>AMRQCAIYGKGGIGKSTTTQNLVAALAEMGKKVMIVGCDPKADSTRLILHSKAQNTIMEMAAEAGTVEDLELEDVLKAGYG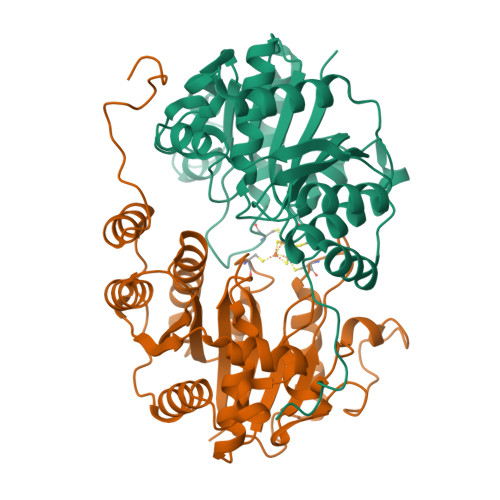GVKCVESGGPEPGVGCAGRGVITAINFLEEEGAYEDDLDFVFYDVLGDVVCGGFAMPIRENKAQEIYIVCSGEMMAMYAANNISKGIVKYANSGSVRLGGLICNSRNTDREDELIIALANKLGTQMIHFVPRDNVVQRAEIRRMTVIEYDPKAKQADEYRALARKVVDNKLLVIPNPITMDELEELLMEFGIMEVEDESIVGKTAEEV[2x]Lamins represent a distinct class within the intermediate filament (IF) protein family. Lamin A (LA) and its splice variant lamin C as well as two closely related lamins B1 and B2 jointly form the lamina, a meshwork of ~3.5-nm-thick filaments located at the inner side of the nuclear envelope. Like for the whole IF family, the basic constitutive unit of the lamin filament is a rod-like dimer which results from a parallel coiled-coil (CC) structure. In line with this, the primary structure of lamins reveals a central α-helical domain responsible for the CC formation which is flanked by non-helical N- and C-terminal domains called the head and the tail respectively.

Three N-terminal constructs incorporated residues 1–70, 17–70 and 22–70 of human LA respectively, fused to residues 215–251 of the Eb1 protein (C-terminal cap). These constructs correspond to the complete or truncated LA head domain followed by the complete coil1A segment (predicted to start with residue 27 and end with residue 67) and the first three residues of linker L1. In contrast, the 1-70-Eb1 structure features an opened-up, ‘unzipped’ coil1A segment, even though the presence of the Eb1 cap keeps the two chains together at the C-terminus. The observed unzipping is especially interesting with respect to the possible mechanism of longitudinal IF assembly. The large differences observed in the dimer structure and crystal lattice contacts between the LA 17-70-Eb1 and LA 1-70-Eb1 structures are most likely due to the different crystallization conditions, rather than a consequence of the complete head being retained in the latter case. Indeed, since the head domain in the LA 1-70-Eb1 structure is almost entirely disordered, it does not seem likely that it plays a major role in the formation of the antiparallel overlap of two coil1A dimers. At the same time, the observed structure clearly reveals the weakness and plasticity of the N-terminal part of coil1A. In fact, the N-terminal opening-up of coil1A dimer is the most pronounced in the LA 1-70-Eb1 structure, followed by a smaller opening in the vimentin structure and a completely regular CC geometry in the 17-70-Eb1 construct.

> RITRLQEKEDLQELNDRLAVYIDRVRSLETENAGLRLRITESEEVVDFYFGKLRNIELICQENEGENDPVLQRIVDILYATDE;> ITRLQEKEDLQELNDRLAVYIDRVRSLETENAGLRLRITESEEVVDFYFGKLRNIELICQENEGENDPVLQRIVDILYATD>GSNRTLIVTTILEEPYVMYRKSDKPLYGNDRFEGYCLDLLKELSNILGFLYDVKLVPDGKYGAQNDKGEWNGMVKEL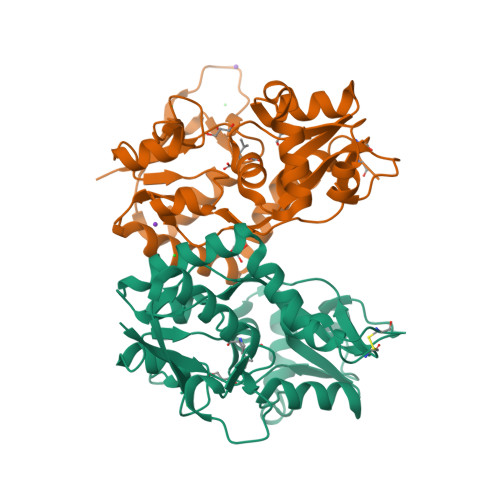IDHRADLAVAPLTITYVREKVIDFSKPFMTLGISILYRKGTPIDSADDLAKQTKIEYGAVRDGSTMTFFKKSKISTYEKMWAFMSSRQQSALVKNSDEGIQRVLTTDYALLMESTSIEYVTQRNCNLTQIGGLIDSKGYGVGTPIGSPYRDKITIAILQLQEEGKLHMMKEKWWRGNGCPE[2x]To gain further insight into the structural conversions in pore formation, we chose pleurotolysin (Ply), a MACPF protein consisting of two components, PlyA and PlyB, from Pleurotus ostreatus. Previous studies have shown that PlyA binds membranes and is required to recruit the pore-forming MACPF protein PlyB to the membrane surface. PlyA and PlyB together form relatively small and regular pores in liposomes. The membrane attack complex/perforin-like family (MACPF) proteins form the largest superfamily of pore-forming proteins identified to date.

Oxidised TMH1 variant PlyBF138C,H221C (TMH1 lock) possessed no detectable lytic activity, but reduction of the disulphide restored wild type lytic activity. Furthermore, the oxidised form could assemble into oligomeric prepores on erythrocytes or liposomes, and these prepores could be converted into lytic pores by disulphide reduction. These data suggest that the TMH1 lock prepore structure is an intermediate in the formation of the pore. Remarkably, the cryo-EM 3-D structure of the TMH1 lock prepore showed that the central sheet of the MACPF domain in the prepore assembly had opened substantially (53° ± 9°). In these prepores, the top half of the barrel has formed, but not the lower, transmembrane part. Indeed, no density could be observed for most of TMH1 and TMH2 and it appears that these regions are largely unstructured. Thus, these data reveal that locking TMH1 has little effect in limiting the MACPF β-sheet opening.

>AYAQWVIIIIHNVGSKDVKIKNLKPSWGKLHADGDKDTEVSASKYEGTVIKPDEKLQINACGRSDAAEGTTGTFDLVDPADGDKQVRHFYWDCPWGSKTNTWTVSGSNTKWMIEYSGQNLDSGALGTITVDTLKK[2x];> SQAGDTLNDVIQDPTRRNKLINDNNLLKGIIMGRDGPVPSSRELIVRPDTLRAIINNRATIETTTMKSMYTSSRYLFPQGRIDFTTPDSGFDDVIKLSPQFTSGVQAALAKATGTEKREALQNLFQEYGHVFRTKVHIGGVLSAHTMETFSKLNVKYIVNGGDYTKIQNTEEWVASTNQSEHWRVIEVTEVTAVADLLPQPIRGQVKDLLKPLLGKWVDVEKVPGLESLPVSVYRPKGAIPAGWFWLGDTADASKALLVKPTLPARSGRNPALTSLHQGSGMTEQPFVDLPQYQYLSTYFGSFAHDTPPGSTLRGLRPDHVLPGRYEMHGDTISTAVYVTRPVDVPFPEDECFDLKSLVRVKLPGSGNPPKPRSALKKSMVLFDSGEK> MHHHHH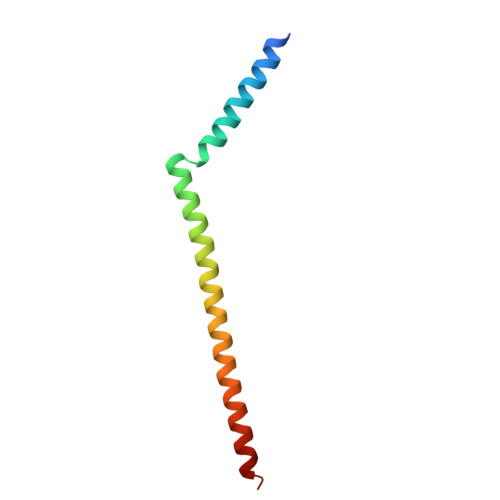HQKLSARLRALRQRQLDRAAAAVEPDVVVKRQEALAAARLKMQEELNAQVEKHKEKLKQLEEEKRRQKIEMWDSM> GPDEEPEEPGRRGSFVEMVDNLRGKSGQGYYVEMTVGSPPQTLNILVDTGSSNFAVGAAPHPFLHRYYQ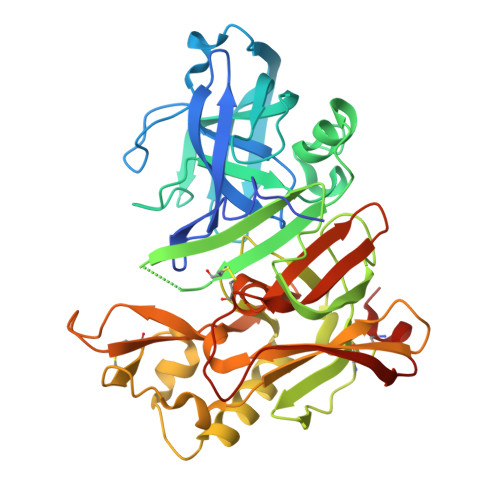RQLSSTYRDLRKGVYVPYTQGKWEGELGTDLVSIPHGPNVTVRANIAAITESDKFFINGSNWEGILGLAYAEIARPDDSLEPFFDSLVKQTHVPNLFSLQLCGAGFPLNQSEVLASVGGSMIIGGIDHSLYTGSLWYTPIRREWYYEVIIVRVEINGQDLKMDCKEYNYDKSIVDSGTTNLRLPKKVFEAAVKSIKAASSTEKFPDGFWLGEQLVCWQAGTTPWNIFPVISLYLMGEVTNQSFRITILPQQYLRPVEDVATSQDDCYKFAISQSSTGTVMGAVIMEGFYVVFDRARKRIGFAVSACHVHDEFRTAAVEGPFVTLDMEDCGYNIPQTDES> MDSYSITNVKYLDPTELH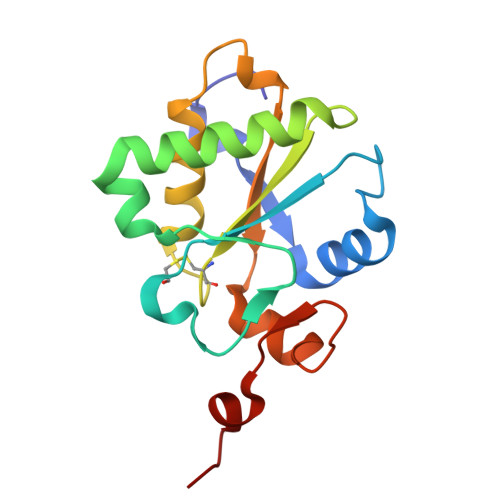RWMQEGHTTTLREPFQVVDVRGSDYMGGHIKDGWHYAYSRLKQDPEYLRELKHRLLEKQADGRGALNVIFHCMLSQQRGPSAAMLLLRSLDTAELSRCRLWVLRGGFSRWQSVYGDDESVTAGYLPDLWRAAAA4-[3-azanyl-6-[1-methyl-5-(1-phenylcyclopropyl)-1,2,4-triazol-3-yl]pyrazin-2-yl]-~{N},~{N}-dimethyl-pyrazole-1-sulfonamide | 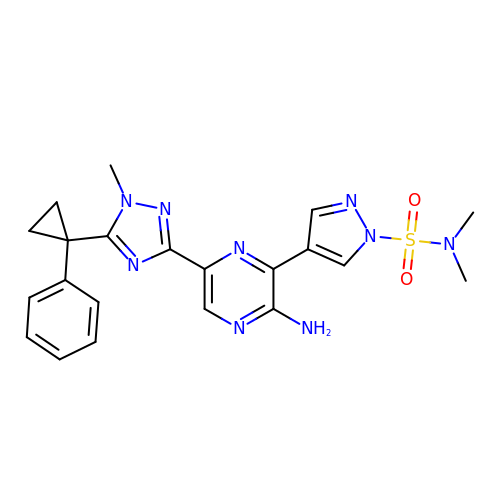C21 H23 N9 O2 S | GMLLOWVABPADNX-UHFFFAOYSA-N>[2x]MPKHEFSVDMTCGGCAEAVSRVLNKLGGVKYDIDLPNKKVCIESEHSMDTLLATLKKTGKTVSYLGLE

Atox1 is a cytosolic small protein (68 amino acids) able to chelate Cu by a conserved surface-exposed Cys-X-X-Cys (CXXC) motif. Once bound to Atox1, Cu is delivered to cytoplasmic metal-binding domains of ATP7A and ATP7B (also called Menkes and Wilson disease proteins, respectively), two homologous multi-domain P1B-type ATPases located in the trans-Golgi network, for incorporation into Cu-dependent enzymes.

For the first time, crystals of Zn-bound human Cu-chaperone Atox1 have been obtained and the structure solved by X-ray diffraction to a resolution of 1.9 Å. The crystals exhibit P65 symmetry and two protein molecules per asymmetric unit (hereinafter named chains A and B). The two chains are equally folded and arranged in a two-fold axis passing through the cage of the metal binding motif, similar to what was found in the previously solved dimeric structures. A positive Fo-Fc electron density signal was found between the two protein chains near the Cys12 and Cys15 residues, supporting the presence of a metal ion. Fortunately, it is possible to confirm the identity and location of a metal ion within a protein by collecting X-ray diffraction data at photon energies close to the metal absorption edge. In our case, a peak in the anomalous scattering density map close to the cysteine residues of the CXXC motifs was found at 9690 eV, an energy right above the Zn K-edge (9640 eV), while no anomalous signal was found close to the Cu K-edge (8970 eV), as shown in Figure 3c. Therefore, it is possible to conclude that the electron density found in between the CXXC metal binding motifs of the two chains belongs to a Zn ion. Zn binds to the sulfur atoms of Cys12 and Cys15 of the two chains in a tetrahedral arrangement, similarly to the Atox1 homodimers formed with other metal ions. The Zn ion presents a crystallographic occupancy of 0.69 and is surrounded by four cysteine residues (Cys12 and Cys15 of chains A and B). The sulfur atoms of the cysteines around the cage are at 2.3–2.4 Å from the metal center and arranged in a tetrahedral geometry, with bond angles ranging from 105° to 118°, as expected for a regular tetrahedral coordination environment. Moreover, although the affinity of Atox1 for Zn2+ is lower than that of EDTA, soaking of the Zn-loaded Atox1 crystals with 2 mM EDTA for 10 min resulted in only limited removal of the metal ion from the coordination cage.>[16x]ETGDKPLGETGTTGFQICKNALKLPVLEVLPGGGWDNLRNVDMGRVMDLTYTNCKTTEDGQYIIPDEVYTIPQKESNLEMNSEVLESWMNYQSTTSLSINTELALFSRVNGKFSTEFQRMKTLQVKDQAVTTRVQVRNRIYTVKTTPTSELSLGFTKALMDICDQLEKNQTKMATYLAELLILNYGTHVITSVDAGAALVQEDHVRSSFLLDNQNSQNTVTASAGIAFLNIVNFKVETDYISQTSLTKDYLSNRTNSRVQSFGGVPFYPGITLETWQKGITNHLVAIDRAGLPLHFFIKPDKLPGLPGPLVKKLSKTVE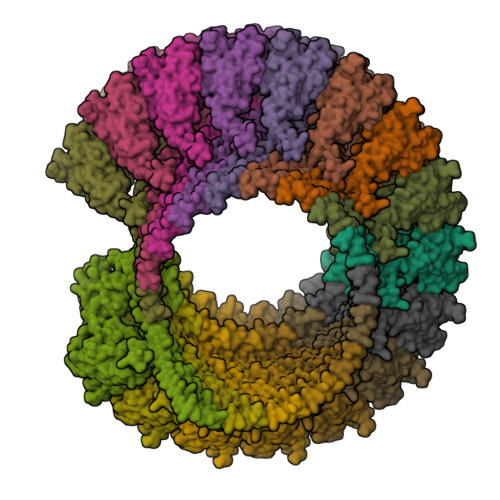TAVRHYYTFNTHPGCTNVDSPNFNFQANMDDDSCDAKVTNFTFGGVYQECTELSGDVLCQNLEQKNLLTGDFSCPPGYSPVHLLSQTHEEGYSRLECKKKCTLKIFCKTVCEDVFRVAKAEFRAYWCVAAGQVPDNSGLLFGGVFTDKTINPMTNAQSCPAGYIPLNLFESLKVCVSLDYELGFKFSVPFGGFFSCIMGNPLVNSDTAKDVRAPSLKKCPGGFSQHLAVISDGCQVSYCVKAGIFTGGSLLPVRLPPYTKPPLMSQVATNTVIVTNSETARSWIKDPQTNQWKLGEPLELRRAMTVIHGDSNGMSGGGTKTETSQVAPA> SNASAFRFGQLALGDRWDIYPQALSRMSREIDKRTSIEAAREPAAVTLSSPTLHETPFLYLAGDREFAIPPEPEVEALRRHLTFGGFLLIDSAEGALGGAFDRSVRRLLQAVFPAPAPGLEIVSGEHVVFKSFYLLERPLGRLALSPVMEGILRDGRLMVA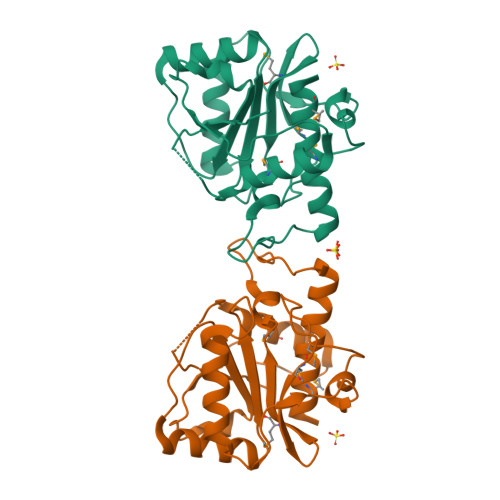YVQNDLGGAFARDDFGNFQLACVPDGERQRELAFRMLVNLVMYALCLD In A. baumannii, the best-characterized multidrug efflux system is the prevalent Acinetobacter drug efflux ABC (AdeABC) tripartite system. This efflux system is capable of mediating resistance to a broad spectrum of clinically relevant antimicrobial agents, such as aminoglycosides, tetracyclines, macrolides, β-lactams, fluoroquinolones, chloramphenicol, and trimethoprim. The AdeABC locus consists of three tandemly linked genes encoding the AdeA periplasmic membrane fusion protein, the AdeB multidrug efflux pump, which is an inner membrane protein belonging to the hydrophobe-amphiphile efflux resistance-nodulation-cell division (HAE-RND) family of efflux transporters, and the AdeC outer membrane channel protein. Each subunit of AdeB contains 12 transmembrane helices (TM1 to TM12) and six periplasmic subdomains (PN1, PN2, PC1, PC2, DN, and DC).

Three distinct conformations of apo-AdeB (AdeB-I, AdeB-II, and AdeB-III) were captured in our cryo-EM data. In the structure of AdeB-I, the three AdeB protomers are identical in conformation, displaying the “extrusion” state of the pump. The periplasmic cleft created by subdomains PC1 and PC2 is closed. An extrusion channel is found in each AdeB protomer. It is interesting that the three AdeB molecules tightly interact with each other, both in the transmembrane and the periplasmic regions, to form a trimer in this state. Within the transmembrane domain, six phosphatidylethanolamine (PE) molecules were observed to bind at the outer leaflet region of the trimeric AdeB pump. Each AdeB protomer forms two distinct PE lipid-binding sites. One of these two binding sites is located at the interior surface of the large central cavity of the trimeric AdeB efflux pump, with each individual AdeB protomer solely responsible for its binding. The other lipid binding site is found within the protomer-protomer interface, where two AdeB protomers interact with each other within their transmembrane regions to anchor this bound PE molecule. It appears that the TM-associated PE molecule may help promote these protomer-protomer interactions within the subunit interface.

>[3x]MSQFFIRRPVFAWVIAIFIIIFGLLSIPKLPIARFPSVAPPQVNISATYPGATAKTINDSVVTLIERELSGVKNLLYYSATTDTSGTAEITATFKPGTDVEMAQVDVQNKIKAVEARLPQVVRQQGLQVEASSSGFLMLVGINSPNNQYSEVDLSDYLVRNVVEELKRVEGVGKVQSFGAEKAMRIWVDPNKLVSYGLSISDVNNAIRENNVEIAPGRLGDLPAEKGQLITIPLSAQGQLSSLEQFKNISLKSKTNGSVIKLSDVANVEIGSQAYNFAILENGKPATAAAIQLSPGANAVKTAEGVRAKIEELKLNLPEGMEFSIPYDTAPFVKISIEKVIHTLLEAMVLVFIVMYLFLHNVRYTLIPAIVAPIALLGTFTVMLLAGFSINVLTMFGMVLAIGIIVDDAIVVVENVERIMATEGLSPKDATSKAMKEITSPIIGITLVLAAVFLPMAFASGSVGVIYKQFTLTMSVSILFSALLALILTPALCATILKPIDGHHQKKGFFAWFDRSFDKVTKKYELMLLKIIKHTVPMMVIFLVITGITFAGMKYWPTAFMPEEDQGWFMTSFQLPSDATAERTRNVVNQFENNLKDNPDVKSNTAILGWGFSGAGQNVAVAFTTLKDFKERTSSASKMTSDVNSSMANSTEGETMAVLPPAIDELGTFSGFSLRLQDRANLGMPALLAAQDELMAMAAKNKKFYMVWNEGLPQGDNISLKIDREKLSALGVKFSDVSDIISTSMGSMYINDFPNQGRMQQVIVQVEAKSRMQLKDILNLKVMGSSGQLVSLSEVVTPQWNKAPQQYNRYNGRPSLSIAGIPNFDTSSGEAMREMEQLIAKLPKGIGYEWTGISLQEKQSESQMAFLLGLSMLVVFLVLAALYESWAIPLSVMLVVPLGIFGAIIAIMSRGLMNDVFFKIGLITIIGLSAKNAILIVEFAKMLKEEGMSLIEATVAAAKLRLRPILMTSLAFTCGVIPLVIATGASSETQHALGTGVFGGMISATILAIFFVPVFFIFILGAVEKLFSSKKKISS>[2x]ECHLSDLLQQLTSVNASKPSERGLVRQEEAEDPACIPIFWVSKWVDYSDKYGLGYQLCDNSVGVLFNDSTRLILYNDGDSLQYIERDGTESYLTVSSHPNSLMKKITLLNYFRNYMSEHLLKAGANITPREGDELARLPYLRTWFRTRSAIILHLSNGTVQINFFQDHTKLILCPLMAAVTYINEKRDFQTYRLSLLEEYGCCKELASRLRYARTMVDKLLSSR;>[2x]LHYPSTTALQE

Polo-like kinase 1 (Plk1) is a well-known mitotic kinase and has been widely reported as a key player in cell division, centrosome maturation, and bipolar spindle formation during multiple stages of mitosis. Plk1 contains an N-terminal catalytic domain and a substrate-binding C-terminal Polo box domain (PBD). The PBD of Plk1 forms a complex through the conserved phospho-Ser/Thr (p-Ser/p-Thr)-binding module of its substrate. Human enhancer filamentation 1 (HEF1, also known as Cas-L or NEDD9) belongs to the Cas scaffold protein family (Efs/Sin and p130Cas/Bcar), which mediates signal transduction through protein-protein interactions.

Two phosphorylated peptides corresponding to 775KVMNSpSNQLC784 and 799LHYPSpTTALQE809 of HEF1, referred to as pSer-780 and pThr-804 peptides, respectively, were synthesized. Each peptide was complexed with Plk1 PBD, and crystallization attempts were made. However, only the Plk1 PBD complexed with pThr-804 peptide gave diffraction quality crystals (see Table 2 and “Experimental procedures” for details). The final model included all Plk1 PBD (residues 371–593) and 800HYPSpTTAL807 of the pThr-804 peptide because the terminal residues were not clearly defined in the electron density maps. There were two copies of the complex in the asymmetric unit of the crystal, which were almost identical, with a root mean square deviation value of 0.36 Å for the 208 Cα atoms. The crystal structure determined at 2.9 Å resolution shows that the pThr-804 peptide is bound in a groove formed by Polo box 1 (PB1; consisting of residues 412–489) and Polo box 2 (PB2; consisting of residues 512–594) of Plk1 PBD. The core of the pThr-804 peptide adopts a β-structure, forming four hydrogen bonds with the last strand of the β-sheet in Polo box 1 of Plk1. In particular, Tyr-801 and Ser-803 of the pThr-804 peptide form hydrogen bonds with the backbone amides and carbonyls of Asp-416 and Trp-414 of Plk1, respectively. The phosphate moiety of the pThr-804 peptide binds to the positively charged binding pocket, forming hydrogen bonds with the side chains of Lys-540 and His-538 of Plk1, and stabilizes the backbone conformation of the peptide by forming hydrogen bonds with the backbone amide of Thr-804. The imidazole ring of His-800 of the pThr-804 peptide is located at the tyrosine cluster of Plk1 PBD and forms hydrogen bonds with Tyr-485, whereas Tyr-801 is on the hydrophobic binding surface formed by Trp-414 and Phe-535 of Plk1. Therefore, the structural analysis clearly suggests that the phosphothreonine at position 804 of HEF1 (pThr-804) plays an important role in specific interaction and recognition by Plk1 PBD.>MAETAPLRVQLIAKTDFLAPPDVPWTTDADGGPALVEFAGRACYQSWSKPNPKTATNAGYLRHIIDVGHFSVLEHASVSFYITGISRSCTHELIRHRHFSYSQLSQRYVPEKDSRVVVPPGMEDDADLRHILTEAADAARATYSELLAKLEAKFADQPNAILRRKQARQAARAVLPNATETRIVVTGNYRAWRHFIAMRASEHADVEIRRLAIECLRQLAAVAPAVFADFEVTTLADGTEVATSP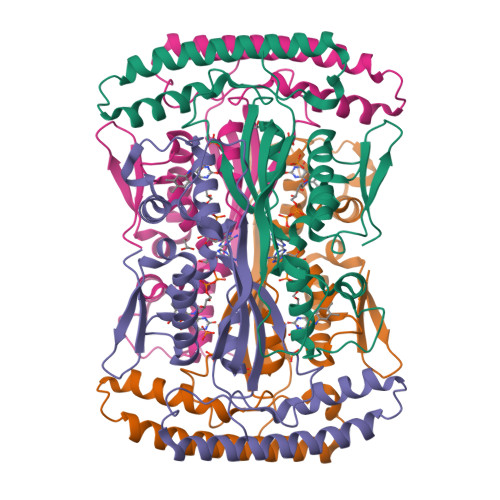LATEALEHHHHHH[4x]>AVSLDRTRAVFDGSEKSMTLDISNDNKQLPYLAQAWIENENQEKIITGPVIATPPVQRLDPGAKSMVRLSTTPDISKLPQDRESLFYFNL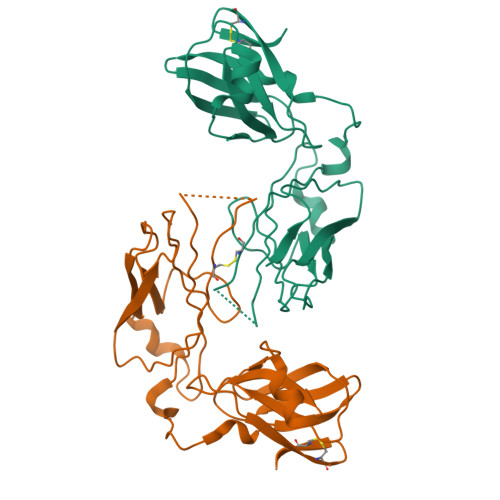REIPPRSEKANVVQIALCTKIKLFYRPAAIKTRPNEVWQDQLILNKVSGGYRIENPTPYYVTVIGLGGSEKQAEEGEFETVMLSPRSEQTVKSANYNTPYLSYINDYGGRPVLSFICNGSRCSVKKEK[2x]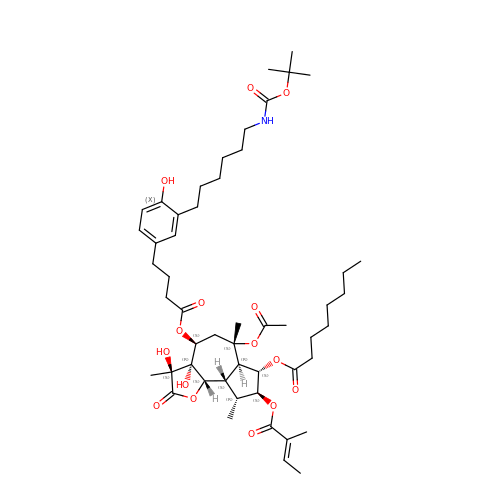(3S,3aR,4S,6S,6aR,7S,8S,9R,9aS,9bS)-6-(acetyloxy)-4-{[4-(3-{6-[(tert-butoxycarbonyl)amino]hexyl}-4-hydroxyphenyl)butanoyl]oxy}-3,3a-dihydroxy-3,6,9-trimethyl-8-{[(2Z)-2-methylbut-2-enoyl]oxy}-2-oxododecahydroazuleno[4,5-b]furan-7-yl octanoate | C51 H77 N O15 | MJLFQZMEQWPDGU-UKQHJVOGSA-N> EDDEDYGDLGGCPFLVAENKTGYPTIVACKQDCNGTTETAPNGTRCFSIGDEGLRRMTANLPYDCPLGQCSNGDCIPKETYEVCYRRNWRDKKNHHHHHH;> MSLAA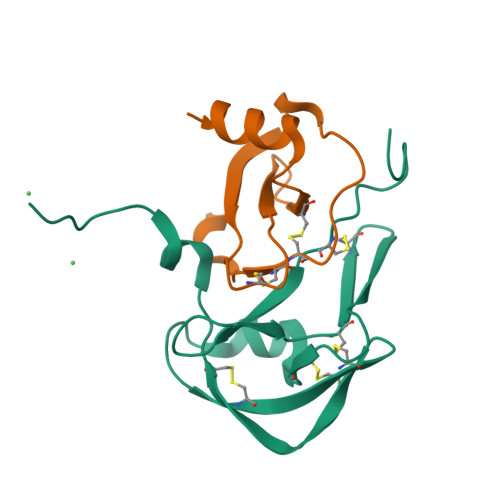DTPTTCCFSYTSRQIPQNFIADYFETSSQCSKPGVIFLTKRSRQVCADPSEEWVQKYVSDLELSA In the barley β-d-glucan glucohydrolase, a glycoside hydrolase family 3 (GH3) enzyme, the Trp286/Trp434 clamp ensures β-d-glucosides binding, which is fundamental for substrate hydrolysis during plant growth and development. HvExoI folds into a two-domain structure consisting of an (α/β)8 barrel (domain 1) and an (α/β)6 sandwich (domain 2) with a 13 Å-deep active site pocket embracing the subsites −1 and +1, positioned at the interface between the two domains. HvExoI catalyses the hydrolytic removal of nonreducing glucose (Glc) moiety from a broad spectrum of poly- and oligomeric β-d-glucosides. The crucial role of substrate binding in HvExoI implies a pair of the aromatic Trp286 and Trp434 residues that form a clamp at the +1 subsite, which is positioned next to a pocket-shaped site at the −1 subsite, housing the Asp285 and Glu491 catalysts.

The well-defined electron density maps of the (1,3)-linked thio-ligands illustrated that the saccharide moieties were attached through the networks of H-bonds formed between nine to ten residues in each case. The W434A mutant was sensitive to 4NP-G3SG and G4SG-OMe, and the data with 4NP-G3SG correlated with substrate specificity and catalytic efficiency. Remarkably, W434A lost all hydrolytic activities with poly- and oligosaccharides, except (1,3)-β-d-linked β-d-glucosides, turning this mutant into a strict (1,3)-β-d-glucosidase, albeit with low specific activities. Conversely, the cluster analysis of the G3OG product in W434A indicated a dramatic shift in poses to ~15% of the populations located in the +1 and +2 subsites, and ~74% to the intermediary (midway) poses at the −1 and +1 subsites.

> HHAADYVLYKDATKPVEDRVADLLGRMTLAEKIGQMTQIERLVATPDVLRDNFIGSLLSGGGSVPRKGATAKEWQDMVDGFQKACMSTRLGIPMIYGIDAVHGQNNVYGATIFPHNVGLGATRDPYLVKRIGEATALEVRATGIQYAFAPCIAVCRDPRWGRCYESYSEDRRIVQSMTELIPGLQGDVPKDFTSGMPFVAGKNKVAACAKHFVGDGGTVDGINENNTIINREGLMNIHMPAYKNAMDKGVSTVMISYSSWNGVKMHANQDLVTGYLKDTLKFKGFVISDWEGIDRITTPAGSDYSYSVKASILAGLDMIMVPNKYQQFISILTGHVNGGVIPMSRIDDAVTRILRVKFTMGLFENPYADPAMAEQLGKQEHRDLAREAARKSLVLLKNGKTSTDAPLLPLPKKAPKILVAGSHADNLGYQCGGWTIEAQGDTGRTTVGTTILEAVKAAVDPSTVVVFAENPDAEFVKSGGFSYAIVAVGEHPYTETKGDNLNLTIPEPGLSTVQAVCGGVRCATVLISGRPVVVQPLLAASDALVAAWLPGSEGQGVTDALFGDFGFTGRLPRTWFKSVDQLPMNVGDAHYDPLFRLGYGLTTNATKKY>[2x]LLVTPPKALLKPLSIPNQLLLGPGPSNLPPRIMAAGGLQMIGSMSKDMYQIMDEIKEGIQYVFQTRNPLTLVISGSGHCALEAALVNVLEPGDSFLVGANGIWGQRAVDIGERIGARVHPMTKDPGGHYTLQEVEEGLAQHKPVLLFLTHGESSTGVLQPLDGFGELCHRYKCLLLVDSVASLGGTPLYMDRQGIDILYSGSQKALNAPPGTSLISFSDKAKKKMYSRKTKPFSFYLDIKWLANFWGCDDQPRMYHHTIPVISLYSLRESLALIAEQGLENSWRQHREAAAYLHGRLQALGLQLFVKDPALRLPTVTTVAVPAGYDWRDIVSYVIDHFDIEIMGGLGPSTGKVLRIGLLGCNATRENVDRVTEALRAALQHCPKKK

AGT is a hepatocyte-specific PLP dependent enzyme, belonging to the Fold Type I family, catalysing the transamination reaction between L-alanine and glyoxylate to produce glycine and pyruvate, thus leading to the removal of glyoxylate. AGT normally localises in the peroxisomes and failure of its detoxification role leads to increased levels of oxalate, coming from oxidation of glyoxylate, causing calcium oxalate precipitation in the kidney and urinary tract. Many pathogenic variants of AGT cause PH1 (primary hyperoxaluria type I), a rare autosomal recessive disorder. Our results shows that two forces generated by the salt bridge between the conserved aspartate residue and the pyridine N1 atom, and by the Schiff base linkage act as opposite springs and are responsible for the fine tilting adjustments of the pyridine plane of PLP.

The tetragonal crystal diffracted to 2.5 Å resolution (space group P41212; cell dimensions: a, b, c = 90.7, 90.7, 141.2), while the orthorhombic crystal yielded a high-resolution (1.7 Å) dataset. In particular, only for this high-resolution dataset, no density for the Schiff base linkage between C4′ of PLP and the Nε of Lys-209 was observed and the best ligand to fit the density was 4′-deoxypyridoxine-5′-phosphate (PLR), which is a PLP lacking the aldehyde oxygen on C4′. On the other hand, it is known that radiation damage might reduce the Schiff base linkage and significantly alter the internal aldimine geometry in a PLP dependent enzyme, especially if the initial geometry is distorted. Therefore, a complete X-ray photoreduction of the Schiff base was hypothesized, to relax the geometrical strain of the internal aldimine. A continuous electron density between C4′ and Nε, relative to the Schiff base linkage, was observed only when the model was refined against the early dataset, while no density at all was present in the maps of the late dataset, indicating that the reduction was induced by radiation damage. Consequently, when the Schiff bond is broken, the C4′-Nε distance increases from 1.5 Å, observed in the early structure, to 3.0 Å in the late one, the optimal distance for the 1,3-protortropic shift to occur. In particular the photo-reduced structure (late) shows that, once the Schiff base is reduced, the interaction with Asp-183 alone tilts the cofactor and brings it in a productive distance (about 3 Å) for the subsequent 1,3-prototropic shift to take place.Herein we reveal widespread occurrence of nucleotidyltransferase-encoding genes in phosphonate biosynthesis and characterize two representative enzymes as phosphonate-specific cytidylyltransferases from the Gram-positive actinobacterium A. rimae and the Gram-negative spirochete T. denticola. These enzymes efficiently activate AEP, presumably for subsequent capture by carbohydrate or lipid nucleophiles. As predicted from gene annotations, the overall structure of the enzyme included an N-terminal PntC connected to a C-terminal AEPT domain. Structure determination of PntC from T. denticola (Tde-PntC) and molecular dynamics analyses indicate that PntC selectivity for the smaller AEP substrate is primarily driven by active site steric constraints.

In contrast to Ari-PntC, the larger two-domain protein Tde1415 was readily crystallized to afford a 2.72 Å structure of the apo enzyme and a 1.95 Å structure of the product complex obtained in the presence of CTP and AEP substrates. Strikingly, the presence of two adjacent magnesium ions in the Tde-PntC active site contrasts with the single ion observed in the Spn-LicC complex, and each apo-enzyme has one less metal ion. For example, a two-magnesium mechanism is favored for CMP-Kdo synthetase (KdsB), FomD employs two metals for cytidylyl (S)-2-hydroxypropoylphosphonate hydrolysis, DNA polymerases commonly employ a two-metal ion mechanism with evidence for an additional third divalent metal ion41, and terpene synthases require three metal ions. Overall, in contrast to Spn-LicC, which loses a salt bridge between Arg129 and a metal-coordinating residue Glu216, the metal coordination sphere of Tde-PntC does not undergo major changes upon ligand binding.

>[4x]MIKQAVILAGGLGSRLKDKTKTMPKGFLEIGGTAIVEQSVQKLLAHGIEKIVIGTGHCNEYYDNLAKKYPAIITVKNENYANTGSMGTLEVCASFVNESFLLLESDLIYDSAGLFSLINDERKNLILASGATKSGDEVYLEADEKNCLTGLSKNRDALKNIFGELVGITKLTKSTLDKMCAYAKIHHSDLPKMEYEHALLEAAKTIPVAIKRIEYFVWREIDNEDHLEMAVKNIYPHIVENEKLRAVRREVLLNPGPATTTDSVKYAQVSADICPREKAFGDLMQWLCDELKLFALASETNPDEYETVMFGCSGTGADEVMVSSCVPDTGRLLVIDNGSYGARMAKIADIYKIPMDIFKSSTYEPLDLQKLEAEFATKKYTHLACVYHETTTGLLNPLHIICPMAKKYGMVTIVDAVSAYCGMPMDLKSLGIDFMASTSNKNIQGMAGVGFVICNKAELEKTKDYPMRNYYLNLYDQYAYFAKTHQTRFTPPVQTMYALRQAVLETKQETVQKRYERYTACWNILVAAIKKLGLKMLVKEEHQSHFITAILEPETPKYSFEALHDFAAEHSFTIYPGKLGNIDTFRIANIGDIQPEEMRRFTVKLKEYMNGIGVGVLEHHHHHH SA1388 was predicted to contain a central PII-like domain and two flanking regions, which together belong to the NIF3-like protein family. Overall, the protein is organized into three distinct structural domains with interconnecting topological connectivities. The two NIF3 domains at the N- and C-terminus of the protein (henceforth denoted as NIF3-N and NIF3-C, respectively) have the same overall fold as canonical NIF3-like proteins, with a central 5 stranded mixed β-sheet and a pair of helices on either side. The middle region of the polypeptide (residues 126–236) bulges out between the two NIF3 domains and is structured as a classical PII-like fold with a (β/α/β)2 architecture, confirming our earlier prediction.

The final model of SA1388 (gi:54040095 Swissprot: P67273;) refined to 2.0Å resolution consists of two subunits in the asymmetric unit. One subunit is traceable across the entire length of polypeptide from the N- to the C-terminus (residues 1 to 366) with the exception of a loop region containing 25 residues (168–193) in the central PII domain. In the other monomer, several more residues are disordered (139 – 193). The two SA1388 monomers in the asymmetric unit tightly associate to form a dimer along the sides of the two NIF3 domains opposite to where the PII-domain is located. Further analysis of symmetry mates within the rhombohedral unit cell showed that the individual subunits are organized into hexamers with a cage-like appearance. In SA1388, the two entries to the central hollow space are capped by the two PII domain trimers. We observe clear electron density for two tightly bound metal ions at the junction of the two NIF3 domains in each SA1388 monomer close to the protein surface that face inside the hexameric toroid. The identity of the metal was determined to be zinc, first by an extended X-ray fluorescence scan at synchrotron and was further confirmed by Inductively Coupled Plasma (ICP) atomic emission spectrometry. Additionally, we observe a clear electron density for a ligand of unknown identity in close proximity to the two bound zinc atoms that would provide two additional metal ligands, one to each of the two metal ions to complete the octahedral metal center configuration. By trial and error, we have ruled out all components in the crystallization solution that might have been inadvertently bound either during crystallization or during cryoprotection and therefore conclude that the observed ligand must in fact be an endogenously bound ligand that was co-purified after recombinant overexpression.

>AMDPMKIADLMTLLDHHVPFSTAESWDNVGLLIGDEDVEVTGVLTALDCTLEVVNEAIEKGYNTIISHHPLIFKGVTSLKANGYGLIIRKLIQHDINLIAMHTNLDVNPYGVNMMLAKVMGLKNISIINNQQDVYYKVQTYIPKDNVGPFKDKLSENGLAQEGNYEYCFFESEGRGQFKPVGEANPTIGQIDKIEDVDEVKIEFMIDAYQKSRAEQLIKQYHPYETPVFDFIEIKQTSLYGLGVMAEVDNQMTLEDFAADIKSKLNIPSVRFVGESNQKIKRIAIIGGSGIGYEYQAVQQGADVFVTGDIKHHDALDAKIHGVNLIDINHYSEYVMKEGLKTLLMNWFNIEKINIDVEASTINTDPFQYI[2x]The genus Enterovirus within the Picornaviridae, a family of non-enveloped viruses with a positive single-stranded RNA genome, is comprised of more than 100 serotypes. Human enteroviruses (EV) are presently classified into four groups, Enterovirus A-D (EV-A, B, C, and D), among which EV-B, the largest group, consists of over 60 serotypes, including all 6 serotypes of coxsackievirus B (CVB1-6), coxsackievirus A9 (CVA9), over 30 serotypes of echoviruses and more than 20 newly identified enteroviruses. The capsid proteins (VP1, VP2, and VP3) adopt the classical eight-stranded anti-parallel β-barrel configuration with the N-termini residing inside and the C-termini exposed on the surface. Most of the uncoating receptors bind to the “canyon” sites of the viral particle, dislodging the “pocket factor” in VP1 and subsequently triggering conformational changes of the intact particle to release the genome, albeit that SCARB2 binds EV71 outside the canyon.

Here we report the structural characterizations of E30 E-particle, A-particle and mature virion, among which E-particle and mature virion are compact with fully ordered epitopes, showing the potential to be ideal vaccine candidates. Two fundamental configurations in EVs, the compact form, generally ~160S mature virions (termed “F-particles”) and the expanded state with altered antigenic properties, e.g. ~135S uncoating intermediates (termed “A-particles”) are well documented. Compared to F- and E-particles, the E30 A-particle is markedly expanded with a ~4.5% increase in radius with a maximum diameter of ~345 Å along the fivefold axis. The expansion of the A-particle reflects tectonic movements in the particle, forming perforations at the icosahedral two-fold axes, accompanied by a ~5.5° counterclockwise rotation of the protomeric unit near the threefold axis and a ~7 Å shift away from the two-fold axis of the protomer unit. However, a close examination of the particles reveals that the F-particle differs significantly from the A-particle (RMSD = 1.1 Å in Cα atoms) at the VP1 N-terminus, VP3 GH loop and the A2B loop and C-terminus of VP2. These conformational changes of individual capsid proteins relay a cascade of alterations, separating the α helices of adjacent VP2 subunits and leading to large perforations at the two-fold axes in the A-particle, through which the viral RNA and VP4 might exit. Like most enteroviruses, E30 F-particle possesses the hydrophobic pocket in VP1 harboring a pocket factor, whereas both E- and A-particles lack hydrophobic pocket and harbor no pocket factor.

> NDPESALNRAVGRVADTVASGPVNTEQIPALTAVETGHTSQVVPSDTMQTRHVINYHTRSESSIENFMGRAACVYIAQYATEKVNDELDRYTNWEITTRQVAQLRRKLEMFTYMRFDLEITFVITSSQRTSTTYASDSPPLTHQVMYVPPGGPIPKSYEDFAWQTSTNPSVFWTEGNAPPRMSIPFMSVGNAYCNFYDGWSHFSQSGVYGYTTLNNMGHLYFRHVNKSTAYPVNSVARVYFKPKHVKAWVPRAPRLCPYLKARNVNFNVQGVTESRNKITLDRSTHNPLANT;> SPTVEECGYSDRVRSITLGNSTITTQECANVVVGYGVWPTYLSDHEATAVDQPTQPDVATCRFYTLESVKWESSSAGWWWKFPEALSDMGLFGQNMQYHYLGRTGYTIHVQCNASKFHQGCLLVVCVPEAEMGAATTDHAFNHTKLSNIGQAMEFSAKKSTDQTGPQTAVHNAGMGVAVGNLTIFPHQWINLRTNNSATIVMPYINSVPMDNMYRHYNFTLMVIPFAKLEHSPQASTYVPITVTVAPMCAEYNGLRLAGHQ;> GLPTMNTPGSTQFLTSDDFQSPSAMPQFDVTPEIQIPGQVRNLMEIAEVDSVVPVNNTEGHVNSMEAYRIPVRPQTSSGEQVFGFQLQPGHDSVLKHTLLGEILNYYANWSGSMKLTFMYCGAAMATGKFLIAYSPPGAGVPGSRRDAMLGTHVIWDVGLQSSCVLCVPWISQTNYRYVTSDAYTDAGYITCWYQTSIVTPPDIPTTSTILCFVSACNDFSVRLLRDTPFITQQALFQ>MTGSSHHHHHHSSGKLMYKNIKILVIGAGIAGPAICYWLRRFGFSPVLIEKYASIRKGGQALDVRGIATHIAKEMGIYDQICGMRTRIECGRFVDSSGKVLHEEHGEKFGFRQDDEVEIVRGDLVEILMKTITDIPCYFNQSIISIQQNSDHVTVNFKDGQVEHYDLVIAADGIHSATRRMVFDKNEYQLIHLGAYLSTFTIPNYLNLRHIDLECEANHKLVSINNDNDPEIARAGFMFLSQHILKDIRDEHEQKQFLCDTFRDFGWETQNILNRMSESDDFYFDAITQVKMNSWTKGRIALIGDAGYCPSPLSGQGNNLAFVGAYILAGELKAADGNYMQAFTRYNALLRPFVDANQEFGVWVSKSFLVEDEVSKEIAEERSNRTLALIKSVSNAITLPQYE[4x]

Tetracycline destructases (TDases) are flavin monooxygenases which can confer resistance to all generations of tetracycline antibiotics. Type 2 TDases have thus far been predominantly identified through soil functional metagenomics with one sequence found in the soil-derived human pathogen Legionella longbeachae. These two types differ in their resistance profiles, with type 1 enzymes conferring resistance to all tetracycline antibiotics including third-generation drugs while type 2 enzymes are generally limited to only first- and second-generation tetracyclines. We determined the X-ray crystal structures of two of these new sequences from Legionella species, and confirmed anhydrotetracycline can inhibit these enzymes’ inactivation of tetracycline antibiotics.

Tet(56-2) and Tet(56-3) are most closely related to Tet(56), at 87.4% and 87.9% amino acid identity respectively, and have 88.6% amino acid identity to each other. Tet(56-2) and Tet(56-3) were also identified in the genomes of Legionella species: L. clemsonensis and L. massiliensis, respectively. We determined the X-ray structures of Tet(56-2) at 1.80 resolution with Rfree/Rwork of 17.43/20.93 and Tet(56-3) at 2.39 Å with Rfree/Rwork of 21.69/24.85. The structures of Tet(56-2) and Tet(56-3) show that the FAD binds in an “OUT” conformation, a conformation that was previously confirmed in X-ray structures of other type 2 TDases. The FAD-interacting residues are conserved between both structures. Most residues in the FAD-binding pocket and the substrate/inhibitor binding pocket are conserved across the three Legionella Tet(56) structures. Intriguingly, L181 and T183 in Legionella Tet(56) enzymes are replaced with V181 and A183 in Tet(50). Similarly, the addition of 1 μg/mL anhydrotetracycline reduced the concentration of tetracycline required to inhibit the growth of Tet(56-3) producing E. coli four-fold, from 32 μg/mL to 8 μg/mL. Apparent IC50 values for anhydrotetracycline inhibition of Tet(56-2) and Tet(56-3) were in the low micromolar range (0.3-30 µM) for tetracycline and doxycycline inhibition. Together these results suggest that anhydrotetracycline inhibition is a promising combination therapy against bacteria producing Tet(56-2) and Tet(56-3).O-[2-(1,3-dioxo-1,3-dihydro-2H-isoindol-2-yl)ethyl] 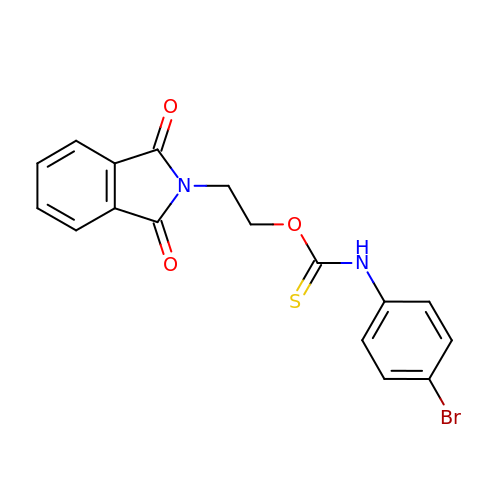(4-bromophenyl)thiocarbamate | C17 H13 Br N2 O3 S | BDVAWAILQCYMQE-UHFFFAOYSA-N>[3x]MMNEKILIVDDQSGIRILLNEVFNKEGYQTFQAANGLQALDIVTKERPDLVLLDMKIPGMDGIEILKRMKVIDENIRVIIMTAYGE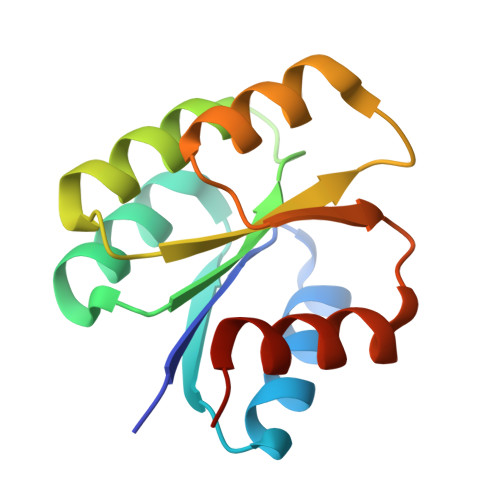LDMIQESKELGALTHFAKPFDIDEIRDAVKKYLPLKSN The ycn operon comprises genes encoding three proteins: the putative copper importer YcnJ, the copper-dependent transcriptional repressor YcnK, and the uncharacterized Domain of Unknown Function 1775 (DUF1775) containing YcnI. The B. subtilis YcnI protein contains a predicted signal sequence N-terminal to the DUF1775 domain, suggesting that endogenously, the DUF1775 domain is localized extracellularly and tethered to the membrane by the C-terminal transmembrane helix. We crystallized both the apo and copper-bound forms of the protein and determined their structures to a resolution of 2.05 and 2.11 Å, respectively. Overall, BsYcnIΔC adopts a cupredoxin fold featuring the characteristic Greek key β barrel shared among many bacterial copper-binding proteins.

The fold of the apo structure of BsYcnIΔC is very similar to that of the Cu-bound protein with an RMSD of 0.59 Å over 127 Cα. The primary differences are in the N-terminal region near the Cu-binding site. Instead of the His27 and Glu50 side chains turning in toward one another as they do in the Cu-bound form, in the apo form, these residues are oriented away from one another with the N terminus directly hydrogen bonding to the side chain of Glu50. In one of the two chains of the asymmetric unit, we observe two alternate conformations for His27, suggesting that this side chain displays a degree of flexibility. In our apo structure, we also observe a malonate molecule from the cryoprotectant solution near the N terminus, indicating that this region of the protein is solvent accessible.

>[2x]HVSVKPAESAAGSWETYTMKVPSEKNLPTTKVVLKMPKDVEFQQYEPIPGWKVSTQKHDDKSVSVTWEATDGGIQEGQFQQFTFVAKNPDKAEEAAWDAYQYYKDGSIVEWTGDEDADTPHSITNITSA>[2x]GPMEEP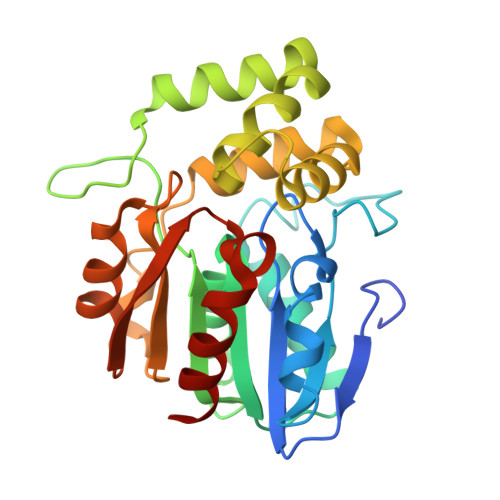SLLDAHNVRVVGMGSELVVLGHGFGTDQSVWKHVIPHLVDDYRVILFDNMGAGTTDPEFFSFSRYSTLHGYADDLLSILEELEVESCIYVGHSVAGMVGCLASLERPEIFTKIITLSASPRYLNDRDYFGGFEQDDLNQLFEAMQSNFKAWVSGFAPLAVGADIDSMAVQEFGRTLFNIRPDIAFSVAKTIFQSDLRIMLPKVTVPCHILQSSKDLAVPLVVADYLHHALGGPTIVEVLPTEGHLPQLSSPDIIIPVLKRHLAGSL>[2x]MGHHHHHHHHHHGASGGGSHMENLYFQGAMPVDLSTTLSWKSATGEAATMLDELQPNILKAHVRDRLTVLFLGFGD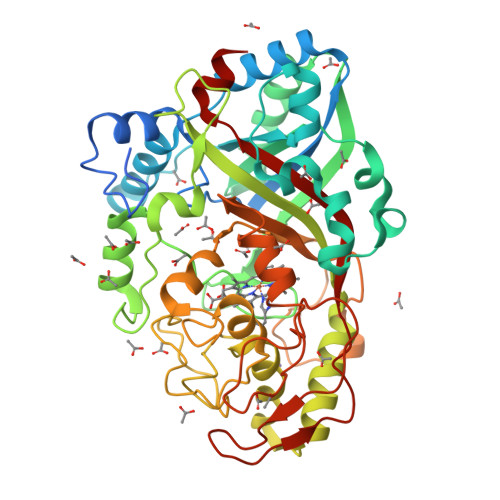AAEARTFLNGLSGLMKSARTHLQEVEAHKLTKAVGTPYLGVGLTAHGYATLGVTAPADPSFTAGAKAAVEKLADPAVTEWEGHYQQTIDAVLLLGDATAGPVRTLRRQVEALRPASVTVVGEESGLGLANANGDGIEHFGYVDGRSQPLFLTEDVDAERDTTDGVNDWDPSAPLEQVLVPDPAAPDPTVHFGSYFVFRKLEQNVRLFKEAERDLAHDLGLRGEDRERAGAMLVGRFEDGTPLTAQSAPGSHHPVGNDFSYDSDKLGQKCPFHAHIRKTNPRGSGGAEAPEEERKHLMARRGQTYGRRHDDPNADLPPRLRPAKDVGLLFMAFNSNLGNQFEFTQQIWANNPAFPFPPDGSQPGLDPVIGQGARAPQKYAPEWGHNNVAEATDPIPQAVTMKGGEYFFMPSLAFLRSL>GMSQLDKDAFEVLLANCADEPIQFPGAIQPHGLLFTLKEPELTILQVSANVQSVLGKVPDQLAGQTLDCVLGAGWAEVIRSTSANDSLVDVPRLLMSVEGVEFEALLHRSQEALVLELEIQDKAAQAISYSERTGNMGRMLRQLHAAADLQTLYEVSVREIQRMTGYDRVLIYRFEEEGHGQVIAEASAPAMELFNGLFFPASDIPEQARELYRRNWLRIIPDANYTPVPLVPQLRPDTQQQLDLSFSTLRSVSPIHCQYMKNMGVLSSMSVSLIQGGKLWGLISCGHRTPLYVSHELRSACQAIGQVLSLQISAMEALEVSRQRETKIQTLQQLHQMMATSDTDVFDGLAQQPQLLMDLVGATGVAIIEDRQTHCYGNCPEPSDIRALHTWMMAGGEPVYASHHLSSVYPPGEAYQTLASGVLAMSLPKPVDNGVIWFRPEVKQSVQWSGDPNKPLNLDASDNTLRLQPRTSFEIWKVEMTGIATKWSHGDVFAANDLRRSALENDLARQVSKEQQAVRARDELVAVVSHDLRNPMTVISMLCGMMQKSFSSDGPHTSRRISTAIDTMQQAASRMNVLLEDLLDTSKIEAGRYTITPQPLEVSQIFEEAYTLLAPLAMDKSIEISFNAEPDIKVNADPERLFQVLSNLIGNAIKFTPKLGRIGVAAMSNGDEVVFTVRDSGEGIPPEQLPHIFERYWTVKEGNPTGTGLGLYISQGIIKAHGGELAAQSQVGHGSEFRFTVPIAH[2x]

Phytochromes (Phys) are a divergent cohort of bili-proteins that detect light through reversible interconversion between dark-adapted Pr and photoactivated Pfr states. Here, we present models of both states for a dimeric Phy with histidine kinase (HK) activity from the proteobacterium Pseudomonas syringae, which were built from high-resolution cryo-EM maps (2.8–3.4-Å) of the photosensory module (PSM) and its following signaling (S) helix together with lower resolution maps for the downstream output region augmented by RoseTTAFold and AlphaFold structural predictions. Pr/Pfr comparisons show that bilin phototransformation alters PSM architecture culminating in a scissoring motion of the paired S-helices linking the PSMs to the HK bidomains that ends in reorientation of the paired catalytic ATPase modules relative to the phosphoacceptor histidines. This action apparently primes autophosphorylation enroute to phosphotransfer to the cognate DNA-binding response regulator AlgB which drives quorum-sensing behavior through transient association with the photoreceptor.

From PsBphP1 preparations dissolved in a HEPES-NaOH (pH 7.5) buffer containing 175 mM KSCN, we generated cryo-EM maps of Pr and Pfr using either dark-adapted samples containing solely Pr or samples irradiated to steady state levels of Pfr (~80% of total Phy pool) with red light immediately before freezing. The combined averages then generated an EM density map of the PSM at 2.9-Å resolution which was further improved to 2.8-Å resolution through symmetry expansion and local refinement of 1,666,098 matching protomers. The resulting data allowed construction of a head-to-head dimeric model encompassing residues 12-459 and 466-516 of protomer A and residues 11-459 and 466-516 of protomer B. While this 3D map provided high resolution for the PSMs, the HK bidomains and much of the S-helices were poorly visible probably due to high mobility. BV was covalently linked via a thioether linkage to Cys16 within the NTE. As expected from other homodimeric Pr models, BV in both protomers assumed a ZZZssa configuration, and was fixed within the GAF domain pocket by an extensive network of conserved amino acid contacts to all four pyrrole rings and the B- and C-ring propionates. Besides the covalent connection, the PAS and GAF domains were tightly linked non-covalently via hydrophobic interactions within the figure-of-eight knot created by a lasso loop extending from the GAF domain to tether the N-terminal extension (NTE) projecting from the PAS domain, which was further solidified by a noncovalent contact involving Ile27 at the knot center. The GAF and PHY domains in PsBphP1 as Pr were linked covalently via the intervening helical spine and noncovalently through the hairpin extension from the PHY domain contacting the GAF domain near the chromophore.> GAQTTDPNQLKNEGNDALNAKN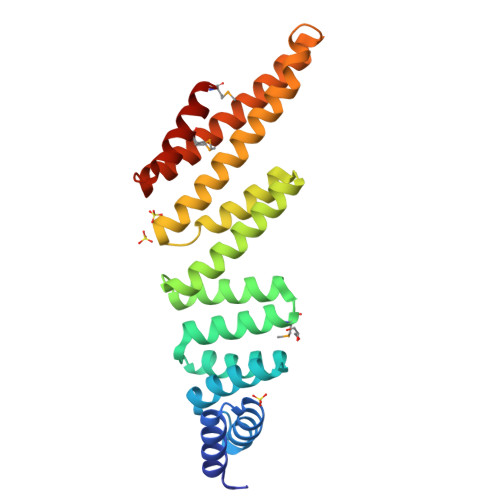YAVAFEKYSEYLKLTNNQDSVTAYNCGVCADNIKKYKEAADYFDIAIKKNYNLANAYIGKSAAYRDMKNNQEYIATLTEGIKAVPGNATIEKLYAIYYLKEGQKFQQAGNIEKAEENYKHATDVTSKKWKTDALYSLGVLFYNNGADVLRKATPLASSNKEKYASEKAKADAAFKKAVDYLGEAVTLSPNRTEIKQMQDQVKAMIK> GAMSGETLLLDYGSGGRASHRLISDLFLRHFDNPILGTLNDAARLDLTGPLAMSTDSYTVDPIFFPGGDIGTLAVHGTVNDVSMLGARPRYLSCGFILEEGLDMDILERVVASMGKAAREAGVFIVTGDTKVVPRGACDKMFINTTGIGEILVDPAPSGDRARPGDAILISGSMGDHGLTILSQRQGLNFAADVCSDSASLNRVVEKLVLEVGDIHVLRDPTRGGLATTLNEIAGQSQAVCHVLETAVPVRESVRNGCSFLGLDPLYLANEGKLICILPEERAEAALAVLREGPHGEHAARIGSVKS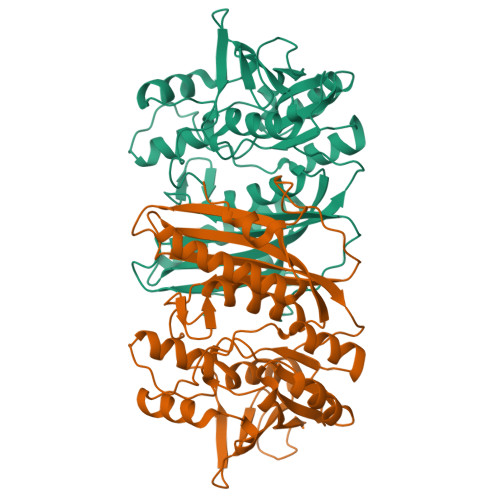VGELGAARAGQVVMETALGGHRLLSMLEGEQLPRIC> KQIADSLSIPPVKAGAKQLPMPSVSGAQIKLLGADYEQLVNSKGKIAPVIS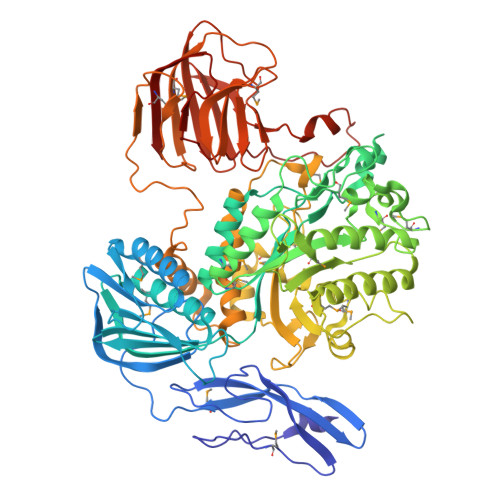DTPVNVSFKVTKDGKEAVSKDYEIMLQAPQAAQGNPKPRIIPEILQWKGGQGEYKLGNTVTIACPDKELGKLFAADMEDVLGKKVKLVAPGAKADISLSLLKGGNLGREGYRLQIARDGVRLGAAAPTGLFWGTRTLLQMLRQTPGSVPCGTAVDFPRYQLRGFMLDVARTPYPLSYLKDVIRTMAWYKMNDLHLVINNNYIFHEHYVDNGHDPFKESYAAFRLESKMKGKDGTPLTARDLFYTKKEFADLVSYARKYGVNIVPEFDTPGHALSFTRLRPDLIYKGPMNHEKRRCEMLDAANPETIDLVSKVFDEYMLKDPKLGRPVFADCGVVHVGADEFYGDKEDYRHFANAVLTHALKRGYTPRIWGSLSAKPGKTPVVSKGVQMNLWSTGWMKAWEAVNQGYDVINTNDGALYIVPFAGYYRMDRNHKGLYNNWIPNRIGNETLPSGHPQLLGGTFAVWNDETDIMHTGYAPYDIWGIISGSMDVLSQKLWGTAKAPDTFEQHRELVSSIGNAPRTNPLHKWKDSQPLTVKPSSLPQKLDKPALGPNYRLTMELELTAAPEGKEQVLLAAPEGELLAVMKDGTVGFRRDDSLEFSFGAKLPVGKKVKVEIVGEPEKTSLLLDGEPAGTAVLKNFSDKSKDFSDKFKHRPKVHRSTFILPLKELGSSFQGKVFHMNVQPL> GSHMKNSVSVDLPGSMKVLVSKSSNADGKYDLIATVDALELSGTSDKNNGSGVLEGVKADASKVKLTISDDLGQTTLEVFKSDGSTLVSKKVTSKDKSSTEEKFNEKGEVSEKIITRADGTRLEYTGIKSDGSGKAKEVLKGYVLEGTLTAEKTTLVVKEGTVTLSKNISKSGAVSVELNDTDSSAATKKTAAWNSGTSTLTITVNSKKTKDLVFTSSN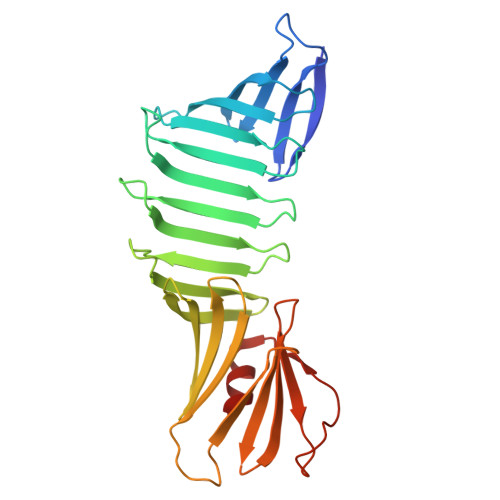TITVQQYDSNGTSLEGSAVEITKLDEIKNALK>[2x]MGSSHHHHHH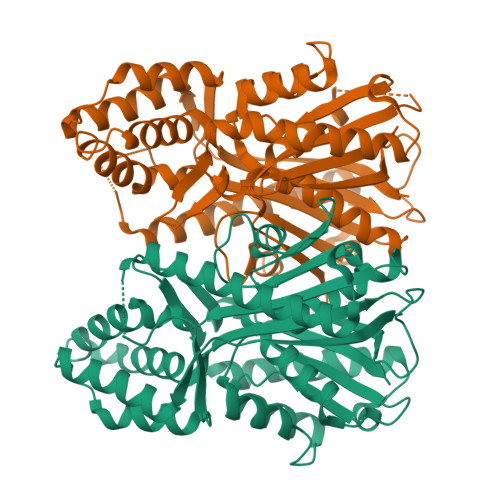SSGENLYFQGHMTYIVSTSTAFPENYYPQTVLAAALRRFFTVMELDFDLEQIDRFFTNVKIDGRYFALPLDSLLDPPTWGVSISRGLENSLNLAETAITKLLEKTNVQPQDISLLASVSMTPAIPSLDGRLMNRIPFSSTLKRLPMNGVGCMGGAFGISRVADYLKAHPKEAAILFAVEISSALWQGSLQANLTSLIRRLPENPSLYSEIIMDIITAALFADGCGAVLMVGKEHPLAKSGLPQVIDNRSFLVPNTVELMGLDVVDNGFRNILRPEVSDALKQGLRPLINGLLADNNIESENLYRWIVHPGGPKVIDTVEAEFGLDSQTLQLSRDTLAEVGNISSATVLYMLDKVLSEEQSPPDSYGLIVAMGPGLAQEAILLKW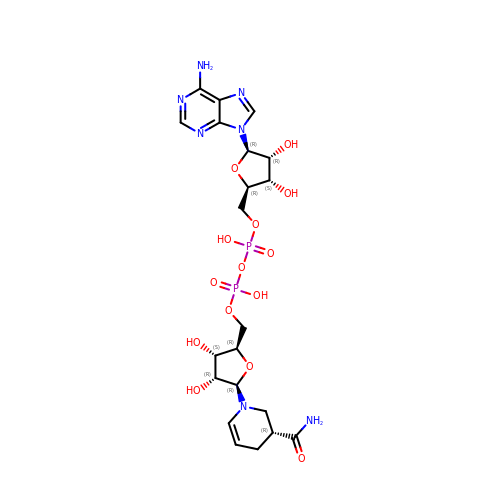[[(2R,3S,4R,5R)-5-[(3R)-3-aminocarbonyl-3,4-dihydro-2H-pyridin-1-yl]-3,4-bis(oxidanyl)oxolan-2-yl]methoxy-oxidanidyl-phosphoryl] [(2R,3S,4R,5R)-5-(6-aminopurin-9-yl)-3,4-bis(oxidanyl)oxolan-2-yl]methyl phosphate | C21 H31 N7 O14 P2 | FDIVXUDDFSHSAE-MTKBYBFRSA-L>GSHNMAEMVETVCGPVPVEQLGKTLIHEHFLFGYPGFQGDVTRGTFREDESLRVAVEAAEKMKRHGIQTVVDPTPNDCGRNPAFLRRVAEETGLNIICATGYCYEGEGAPPYFQFRRLLGTAEDDIYDMFMAELTEGIADTGIKAGVIKLASSKGRITEYEKMFFRAAARAQKETGAVIITHTQEGTMGPEQAAYLLEHGADPKKIVIGHMCGNTDPDYHRKTLAYGVYIAFDRFGIQGMVGAPTDEERVRTLLALLRDGYEKQIMLSHNTVNVWLGRPFTL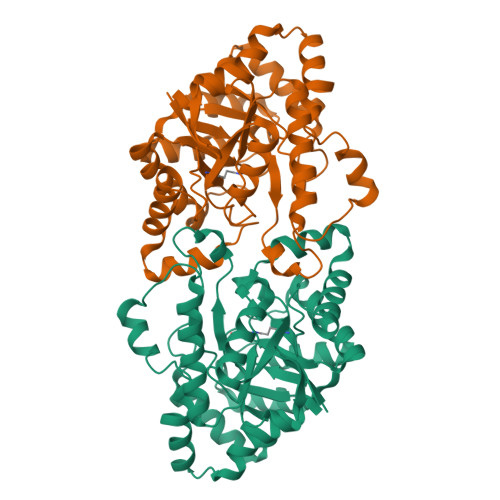PEPFAEMMKNWHVEHLFVNIIPALKNEGIRDEVLEQMFIGNPAALFSA[2x]>[2x]HHHHHHGILMMANRMILNETAWFGRGAVGALTDEVKRRG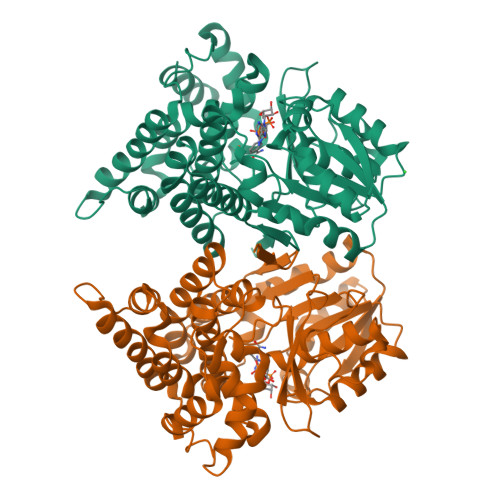YQKALIVTDKTLVQCGVVAKVTDKMDAAGLAWAIYDGVVPNPTITVVKEGLGVFQNSGADYLIAIGGGSPQDTCKAIGIISNNPEFADVRSLEGLSPTNKPSVPILAIPTTAGTAAEVTINYVITDEEKRRKFVCVDPHDIPQVAFIDADMMDGMPPALKAATGVDALTHAIEGYITRGAWALTDALHIKAIEIIAGALRGSVAGDKDAGEEMALGQYVAGMGFSNVGLGLVHGMAHPLGAFYNTPHGVANAILLPHVMRYNADFTGEKYRDIARVMGVKVEGMSLEEARNAAVEAVFALNRDVGIPPHLRDVGVRKEDIPALAQAALDDVCTGGNPREATLEDIVELYHTAW>APSTAGLGYGSWEIDPKDLTFLKELGTGQFGVVKYGKWRGQYDVAIKMIREGSMSEDEFIEEAKVMMNLSHEKLVQLYGVCTKQRPIFIITEYMANGCLLNYLREMRHRFQTQQLLEMCKDVCEAMEYLESKQFLHRDLAARNCLVNDQGVVKVSDFGLSRYVLDDEYTSSVGSKFPVRWSPPEVLMYSKFSSKSDIWAFGVLMWEIYSLGKMPYERFTNSEAAEHIAQGLRLYRPHLASERVYTIMYSCWHEKADER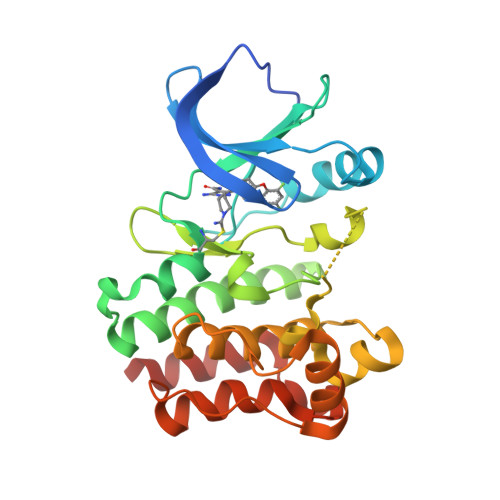PSFKILLSNILDVMDEES[2x]5'-O-(acetylsulfamoyl)adenosine | C12 H16 N6 O7 S | 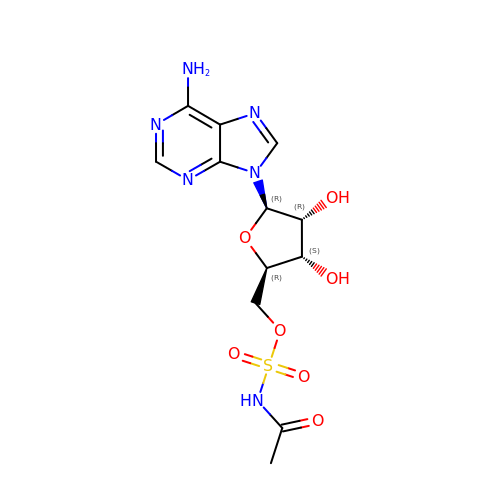SKYBLZMECJREBK-WOUKDFQISA-N N-(2-HYDROXY-4-OXO-BUTYL)-N-(3-OXO-TRANSPROPENYL)AMINE | C7 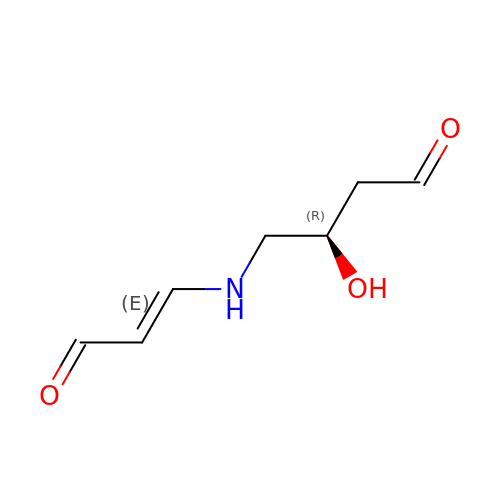H11 N O3 | FXITUJNZFYVSNC-RCYFRSRISA-N> MELKHSISDYTEAEFLQLVTTICNADTSSEEELVKLVTHFEEMTEHPSGSDLIYYPKEGDDDSPSGIVNTVKQWRA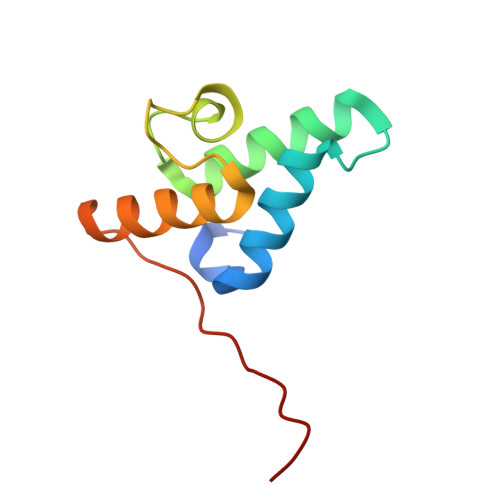ANGKSGFKQGLEHHHHH>GIDPFTK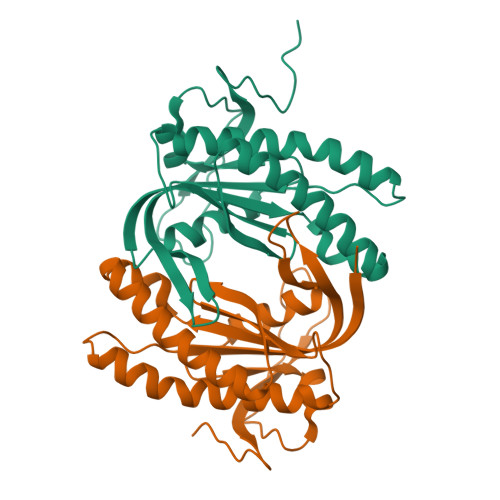MGGDRRPITILTSDLRGFTSTSEGLNPEEVVKVLNIYFGKMADVITHHGGTIDEFMGDGILVLFGAPTSQQDDALRAVACGVEMQLALREVNQQVTGLGLQPLEMGIGINTGEVVVGNIGSEKRTKYGVVGAQVNLTYRIESYTTGGQIFISSTTLEAAGDRVHVNGNRTVQPKGVKDPVVIWDVAGVGEPYNLSLAVEEQ[6x]1-(2-aminoethyl)-3-[2-(quinolin-3-yl)pyridin-4-yl]-1H-pyrazole-5-carboxylic 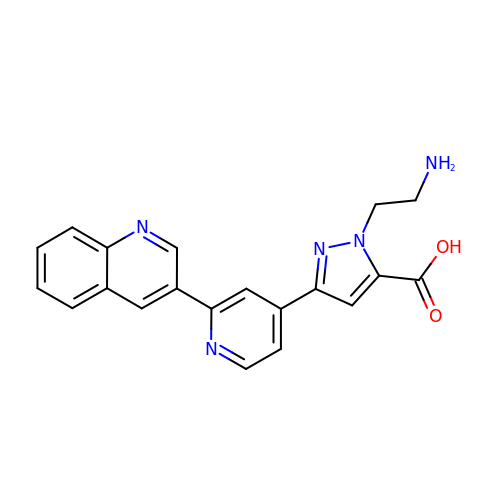acid | C20 H17 N5 O2 | IDPLDWUOSVSMNS-UHFFFAOYSA-N>GMSAKAAEGYEQIEVDVVAVWKEGYVYENRGSTSVDQKITITKGMKNVNSETRTVTATHSIGSTISTGDAFEIGSVEVSYSHSHQKSQVSMTQTEVYSSKVIEHTITIPPTSKFTRWQLNADVGGAGIEYMYLIDEVTPIGGTQSIPQVITSRAKIIVGRQIILGKTEIRIKHAERKEYMTVVSRKSWPAATLGHSKLFKFVLYEDWGGFRIKTLNTMYSGYEYAYSSDQGGIYFDQGTDNPKQRWAINKSLPLRHGDVVTFMNKYFTRSGLCYDDGPATNVYCLDKREDKWILEVVG[18x]

One of the few described eukaryotic members of the aβ-PFT family is lysenin, an invertebrate member present in the earthworm Eisenia fetida. Lysenin is present in the coelomic fluid of earthworms and is produced to act defensively against parasitic microorganisms by forming pores in sphingomyelin (SM)-containing membranes. Monomeric lysenin consists of two distinct domains, the elongated N-terminal domain (pore-forming module, PFM) that shares the fold of all aβ-PFTs, and the C-terminal β-trefoil lectin type domain21. We reveal that lysenin forms pores using nine subunits assembled to form to a large extent a smooth-walled tubular β-barrel structure flanked on the outside by the C-terminal domains.

Based on the crystal structure of the monomeric lysenin, five negative charges were removed from the proposed transmembrane region (Glu84Gln, Glu85Lys, Glu92Gln, Glu97Ser and Asp126Gly) to create the mutant RL1. RL1 still readily forms stable oligomers in the presence of SM-containing membrane and successfully captures and translocates DNA strands under an applied voltage potential. The homogeneous RL1 nonamer was crystalized and its structure determined at 3.1 Å resolution. Two nonameric oligomers were present in the asymmetric unit, packed in a head-to-head manner. The RL1 nonamer reveals a mushroom-shaped transmembrane pore with a central stem built of a long β-barrel. The bottom half of the mushroom cap is composed of the C-terminal domains of each protomer, and the upper part, named the collar, of β-strands originating from the N-terminal domains. The β-barrel is located in the middle of the oligomeric assembly and is built by nine β-hairpins, each resulting from the unfurling of a significant portion of the N-terminal domain of each protomer. The height of the pore is ∼11 nm, of which 10 nm belongs to the β-barrel, with the widest dimension of the cap 12.3 nm. The inner surface of the RL1 channel is mostly polar, with negatively charged residues framing the top and the bottom. If mutated residues in RL1 are modelled back to their wild-type counterparts, the inner surface of the channel becomes almost completely negatively charged, thus neatly explaining the reported exclusivity for the passage of cations as well as the inability of the wild-type lysenin pores to translocate DNA.> MAGSAPLRILVYSDNPRTREQVRLALGKRIHPELPEIEYVDVATAPMAIS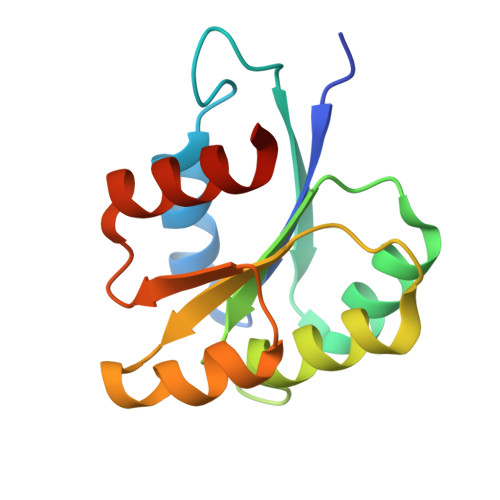QMDAGGFDLAILDGEATPAGGMGVAKQVKDEIDDCPPILVLTGRADDAWLAKWSRAEAAVPHPIDPIRLSDAVVSLLRAPAQ>[4x]SMKAARWHNQKDIRIEHIEEPKTEPGKVKIKVKWCGICGSDLHEYLGGPIFIPVDKPHPLTNETAPVTMGHEFSGEVVEVGEGVENYKVGDRVVVEPIFATHGHQGAYNLDEQMGFLGLAGGGGGFSEYVSVDEELLFKLPDELSYEQGALVEPSAVALYAVRSSKLKAGDKAA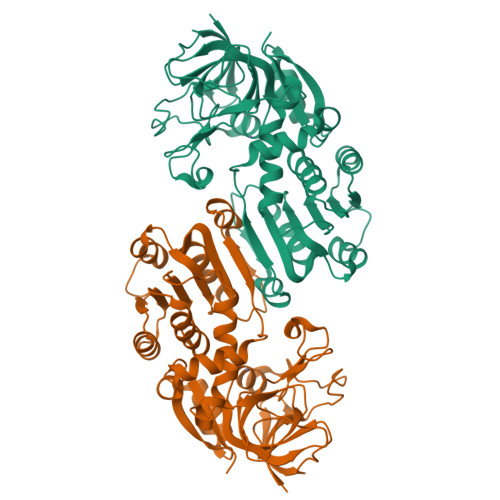VFGCGPIGLLVIEALKAAGATDIYAVELSPERQQKAEELGAIIVDPSKTDDVVAEIAERTGGGVDVAFEVTGVPVVLRQAIQSTTIAGETVIVSIWEKGAEIHPNDIVIKERTVKGIIGYRDIFPAVLSLMKEGYFSADKLVTKKIVLDDLIEEGFGALIKEKSQVKILVRPN> SWDLVT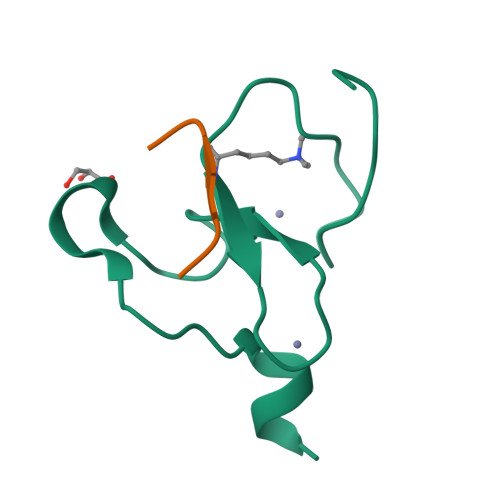CFCMKPFAGRPMIECNECHTWIHLSCAKIRKSNVPEVFVCQKCRDS;> ARTKQTARKST> EPLPPHIIRFNDMAQHLLKKV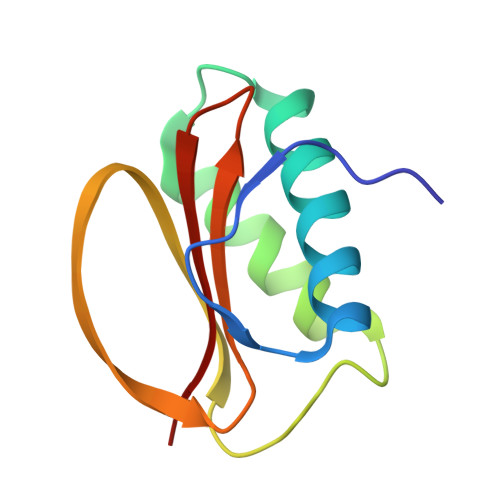IRQADVLIKENPQGLEKDIALNLVKFVKSQPEFKIGDGEWQCIIGKNFGCSLTFDANVLAFFDLLPSRKSILLFKSG> MSEFLTPERTVYDSGVQFLRPKSLDEFIGQENVKKKLSLALEAAKMRGEVLDHVLLAGPPGLGKTTLAHIIASELQTNIHVTSGPVLVKQGDMAAILTSLERGDVLFIDEIHRLNKAVEELLYSAIEDFQIDIMIG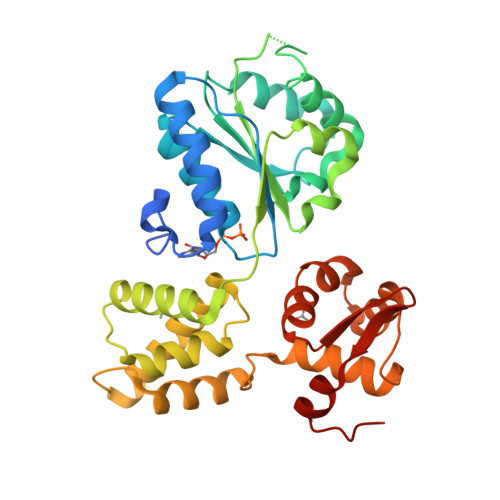KGPSAKSIRIDIQPFTLVGATTRSGLLSSPLRSAFGIILELDFYTVKELKEIIKRAASLMDVEIEDAAAEMIAKRSRGTPRIAIRLTKRVRDMLTVVKADRINTDIVLKTMEVLNIDDEGLDEFDRKILKTIIEIYRGGPVGLNALAASLGVEADTLSEVYEPYLLQAGFLARTPRGRIVTEKAYKHLKYEVPENRLF>[4x]AHHHHHHSSGLEVLFQGPPEGAALTEKTDIFESGRNGNPNKDGIKSYRIPALLKTDKGTLIAGADERRLHSSDWGDIGMVIRRSEDNGKTWGDRVTITNLRDNPKASDPSIGSPVNIDMVLVQDPETKRIFSIYDMFPEGKGIFGMSSQKEEAYKKIDGKTYQILYREGEKGAYTIRENGTVYTPDGKATDYRVVVDPVKPAYSDKGDLYKGDQLLGNIYFTTNKTSPFRIAKDSYLWMSYSD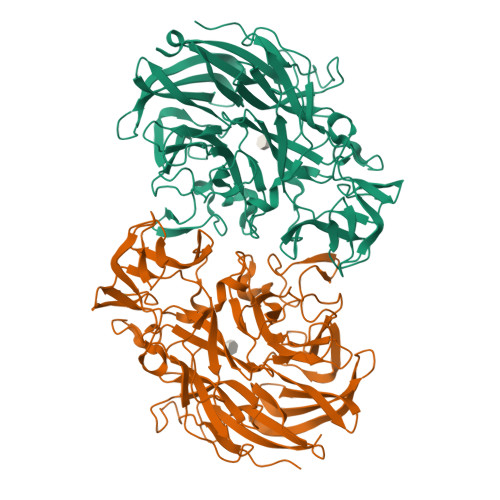DDGKTWSAPQDITPMVKADWMKFLGVGPGTGIVLRNGPHKGRILIPVYTTNNVSHLDGSQSSRVIYSDDHGKTWHAGEAVNDNRQVDGQKIHSSTMNNRRAQNTESTVVQLNNGDVKLFMRGLTGDLQVATSKDGGVTWEKDIKRYPQVKDVYVQMSAIHTMHEGKEYIILSNAGGPKRENGMVHLARVEENGELTWLKHNPIQKGEFAYNSLQELGNGEYGILYEHTEKGQNAYTLSFRKFNWEFLSKN> KLHIPVMVDEVVHCLSPQKGQIFLDMTFGSGGHTKAILQKESDIVLYALDRDPTAYALAEHLSELYPKQIRAMLGQFSQAEALLMKAGVQPGTFDGVLMDLGCSSMQLDTPERGFSLRKDGPLDMRMDGGRYPDMPTAADVVNALDQQALASILRTYGEEKHAKKIASAIVQARSIYPITRTQQLASIVAGAFPPSAIYTRKDLLQRSTHIATKTFQALRIFVNNELNELYTGLKTAQKFLRPGGRLVALSFHSLEDRIVKRFLLGISMTERFNLSVRQQVMKTSQLGSDHENTEEVSMRRAPLMWELIHKKVLSPQDQDVQDNPRGRSAKLRAAIKL

The m4C methyltransferase METTL15 maintains mitochondrial homeostasis by catalyzing m4C839 located in 12 S rRNA helix 44 (h44). Similar to other members of rRNA methyltransferases, METTL15 has a two-domain structure: an MTase domain (domain 1) and a scaffold-like domain (domain 2). The domain 2 of METTL15 contained five α-helices and one η-helix, which formed a scaffold for the binding of RNA substrates or other functional proteins. Here, we reported a series of crystal structures of human METTL15–hsRBFA–h44–SAM analog, METTL15–hsRBFA–SAM, METTL15–SAM and apo METTL15.

To further investigate the mechanism of m4C839 modification, we determined the structures of apo METTL15 and the binary complex METTL15–SAM. Comparison of these two structures revealed that the root-mean-square deviation (r.m.s.d.) of the Cα atom was only 0.145 Å (269 to 269 atoms). Therefore, we mainly used the METTL15–SAM complex for subsequent description. Comparison of the electrostatic potential surface of these two structures showed that the positive charge at the SAM-binding pocket of METTL15 was significantly enriched after SAM binding. The crystal structure was solved by molecular replacement using the structure of apo METTL1570–407 solved previously as the search model.Bromodomains (BRDs) are protein interaction modules that specifically recognize ε-N-lysine acetylation motifs, a key event in the reading process of epigenetic marks. The 61 BRDs in the human genome cluster into eight families based on structure/sequence similarity. Despite large sequence variations, all BRD modules share a conserved fold that comprises a left-handed bundle of four α helices (αZ, αA, αB, αC), linked by loop regions of variable length (ZA and BC loops), which line the Kac binding site and determine binding specificity. The four helices form a deep cavity that is extended by the two loop regions (ZA and BC loops), creating a largely hydrophobic Kac binding pocket.

BRDs are evolutionarily conserved and present in diverse nuclear proteins comprising HATs (GCN5, PCAF), ATP-dependent chromatin-remodeling complexes (BAZ1B), helicases (SMARCA), methyltransferases (MLL, ASH1L), transcriptional coactivators (TRIM/TIF1, TAFs) transcriptional mediators (TAF1), nuclear-scaffolding proteins (PB1), and the BET family (Muller et al., 2011). The most notable structural difference within the BRD core fold is a hairpin insertion located between helix αZ and the ZA loop that is present in all family VIII members. The proximity to the Kac binding site suggests that this insert may play a role in recruitment of acetylated binding partners. The nuclear body protein SP140 as well as the related protein LOC93349 and PCAF showed nonspecific binding to most peptides. In contrast, the second, fourth, fifth, and sixth BRD of PB1, MLL, and TRIM28 interacted with only a few histone Kac peptides.

> SMSPAYLKEILEQLLEAIVVATNPSGRLISELFQKLPSKVQYPDYYAIIKEPIDLKTIAQRIQNGSYKSIHAMAKDIDLLAKNAKTYNEPGSQVFKDANSIKKIFYMKKAEIEHHE> GPLGSIKELAVDEELAAADGLIPRQKSKLCKHGDRGMCEYCSPLPPWDKEYHEKNKIKHISFHSYLKKLNENANKKENGSSYISPLSEPDFRINKRCHNGHEPWPRGICSKCQPSAITLQQQEFRMVDHVEFQKSEIINEFIQAWRYTGMQRFGYMYGSYSKYDNTPLGIKAVVEAIYEPPQHDEQDGLTMDVEQVKNEMLQIDRQAQEMGLSRIGLIFTDLSDAGAGDGSVFCKRHKDSFFLSSLEVIMAARHQTRHPNVSKYSEQGFFSSKFVTCVISGNLEGEIDISSYQVSTEAEALVTADMISGSTFPSMAYINDTTDERYVPEIFYMKSNEYGITVKENAKPAFPVDYLLVTLTHGFPNTDTETNSKFVSSTGFPWSNRQAMGQSQDYQELKKYLFNVASSGDFNLLHEKISNFHLLLYINSLQILSPDEWKLLIESAVKNEWEESLLKLVSSAGWQTLVMILQESG;> GPGHMEPAKLDLPEGQLFFGFPM

Polyubiquitylated proteins in isolation can be direct targets of the proteasome, whereas those embedded into membranes or assembled into multisubunit complexes need to be extracted or segregated by the conserved AAA-family ATPase Cdc48 (yeast) or p97/VCP (metazoan) with the aid of its cofactor complex, Ufd1–Npl4 (UN), prior to the proteasomal degradation. The UN heterodimer is one of the best-characterized cofactors. Here, we present the crystal structures of yeast Npl4 (zf-Npl4-MPN-CTD) in complex with Lys48-linked diubiquitin (K48-Ub2) and with Ufd1 at 2.55 and 1.58 Å resolutions, respectively. The crystal structures reveal that the distal and proximal Ub (Ubdist and Ubprox, respectively) moieties of K48-Ub2 interact with the C-terminal helix and N-terminal loop (N loop) of Npl4 CTD, respectively, and that Ufd1 binds to the groove of Npl4 corresponding to the catalytic groove of JAMM.

To further reveal the structural basis of the interaction between Npl4 and Ufd1, we determined the crystal structure of yNpl4113–580 (E123A K124A E125A) in complex with yUfd1288–305. In the crystal, yNpl4113–580 formed a stoichiometric complex with yUfd1288–305. No large conformational difference was observed between yNpl4113–580 alone and the yUfd1288–305-bound yNpl4113–580. In the complex, residues 298–300 of yUfd1 NBM form a β-sheet with Ins-1 of yNpl4. Leu296, Phe326, Leu353, Met357, Phe419, Pro420, and Tyr424 of yNpl4 form a hydrophobic groove to accommodate Pro289, Leu292, Leu294, Gly297, Leu299, Phe301, Phe303, and Met305 of yUfd1. Gly is more favorable than non-Gly/Pro residues at residue 297. yUfd1 NBM is kinked at Gly297, thereby fitting into the hydrophobic groove in the MPN subdomain of yNpl4. Although the sequence of Ufd1 NBM is variable among eukaryotes, this GxΦxF motif (x and Φ represent any amino acids and hydrophobic amino acids, respectively) is well conserved, reflecting its functional importance. Leu296 and Phe326 of yNpl4 interact with Leu299 and Phe301 of yUfd1, which occupy the third and fifth positions of the GxΦxF motif, and Tyr424 of yNpl4 hydrophobically interacts with the main-chain CO group of Ala290 and the Cα atom of Lys291 in yUfd1. In addition to the hydrophobic interactions, Arg364 and Thr418 of yNpl4 form hydrogen bonds with Glu296 and the main-chain NH group of Ala290 in yUfd1, respectively. However, the present yNpl4113–580–yUfd1288–305 structure reveals that the groove of the MPN domain accommodates yUfd1 NBM.> FFSHWTSKYKERNPTEIAYSEDIERIIDSLVTDEITKEEIIHFLFGNFCFHIETMNDQHIADKFKGYQSSCINLKIEPKVDLADLKDHLIQKQQIWESLYGKHLEKIMLRIREKKKKEKEIPDITTAFNQNAAEYEEKYPNCFTNDLSETKTNFSMTWSPSFEKIELSSEVDYNNAIINKFRESFKSSSRVIYNSPYSSINNQTNKARDITNLVRLCLTELSCDTTKMEKQELEDEIDINTGSIKVERTKKSKEWNKQGSCLTRNKNEFCMKETGRENKTIYFKGLAVMNIGMSSKKRILKKEEIKERISKGLEYDTSERQADPNDDYSSIDMSSLTHMKKLIRHDNEDSLSWCERIKDSLFVLHNGDIREEGKITSVYNNYAKNPECLYIQDSVLKTELETCKKINKLCNDLAIYHYSEDMMQFSKGLMVADRYMTKESFKILTTANTSMMLLAFKGDGMNTGGSGVPYIALHIVDEDMSDQFNICYTKEIYSYFRNGSNYIYIMRPQRLNQVRLLSLFKTPSKVPVCFAQFSKKANEMEKWLKNKDIEKVNVFSMTMTVKQILINIVFSSVMIGTVTKLSRMGIFDFMRYAGFLPLSDYSNIKEYIRDKFDPDITNVADIYFVNGIKKLLFRMEDLNLSTNAKPVVVDHENDIIGGITDLNIKCPITGSTLLTLEDLYNNVYLAIYMMPKSLHNHVHNLTSLLNVPAEWELKFRKELGFNIFEDIYPKKAMFDDKDLFSINGALNVKALSDYYLGNIENVGLMRSEIENKEDFLSPCYKISTLKSSKKCSQSNIISTDEIIECLQNAKIQDIENWKGNNLAIIKGLIRTYNEEKNRLVEFFEDNCVNSLYLVEKLKEIINSGSITVGKSVTSKFIRNNHPLTVETYLKTKLYYRNNVTVLKSKKVSEELYDLVKQFHNMMEIDLDSVMNLGKGTEGKKHTFLQMLEFVMSKAKNVTGSVDFLVSVFEKMQRTKTDREIYLMSMKVKMMLYFIEHTFKHVAQSDPSEAISISGDNKIRALSTLSLDTITSYNDILNKNSKKSRLAFLSADQSKWSASDLTYKYVLAIILNPILTTGEASLMIECILMYVKLKKVCIPTDIFLNLRKAQGTFGQNETAIGLLTKGLTTNTY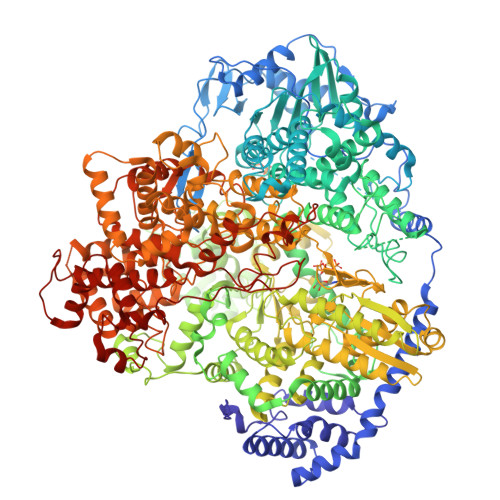PVSMNWLQGNLNYLSSVYHSCAMKAYHKTLECYKDCDFQTRWIVHSDDNATSLIASGEVDKMLTDFSSSSLPEMLFRSIEAHFKSFCITLNPKKSYASSSEVEFISERIVNGAIIPLYCRHLANCCTESSHISYFDDLMSLSIHVTMLLRKGCPNEVIPFAYGAVQVQALSIYSMLPGEVNDSIRIFKKLGVSLKSNEIPTNMGGWLTSPIEPLSILGPSSNDQIIYYNVIRDFLNKKSLEEVKDSVSSSSYLQMRFRELKGKYEKGTLEEKDKKMIFLINLFEKASVSEDSDVLTIGMKFQTMLTQIIKLPNFINENALNKMSSYKDFSKLYPNLKKNEDLYKSTAKNLKIDEDAILEEDELYEKIASSLEMESVHDIMIKNPETILIAPLNDRDFLLSQLFMYTSPSKRNQLSNQSTAKLALDRVLRSKARTFVDISSTEKMTYEENMEKKILEMLKFDLDSYCSFKTCVNLVIKDVNFSMLIPILDSAYPCESRKRDNYNFRWFQTEKWIPVVEGSPGLVVMHAVYGSNYIENLGLKNIPLTDDSINVLTSTFGTGLIMEDVKSLVKGKDSFETEAFSNSNECQRLVKACNYMIAAQNRLLAINTCFTRKSFPFYSKFNLGRGFISNTLALL HOMOTROPINE | C16 H21 N O3 | 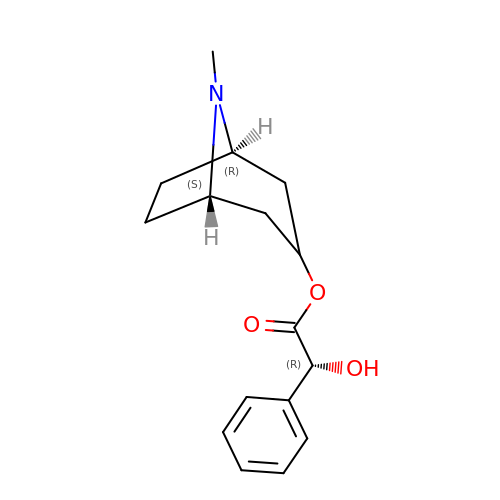ZTVIKZXZYLEVOL-LXTVHRRPSA-N> DLADRFAELERRYDARLGVYVPATGTTAAIEYRADERFAFCSTFKAPLVAAVLHQNPLTHLDKLITYTSDDIRGISPVAQQHVQTGMTIGQLCDAAIRYSDGTAANLLLADLGGPGGGTAAFTGYLRSLGDTVSRLDAEESELNRAPPGDERDTTTPHAIALVLQQLVLGNALPPDKRALLTDWMARNTTGAKRIRAGFPADWKVIDKTGTGGYGRANDIAVVWSPTGVPYVVAVMSDRAGGGYDAEPREALLAEAATCVAGVLA

BlaC is a class A serine β‐lactamase found in Mycobacterium tuberculosis (Wang et al., 2006). The enzymes in this class utilize an active site serine (Ser70) to perform a nucleophilic attack on β‐lactam rings, forming a covalent acyl‐enzyme intermediate that is subsequently hydrolyzed (Fisher & Mobashery, 2009; Strynadka et al., 1992). BlaC can efficiently hydrolyze penicillin antibiotics but has low activity against later‐generation oxyimino‐cephalosporins, such as ceftazidime, due to their bulky C7β aminothiazole‐oxyimino side chain (Sun et al., 2023; Wang et al., 2006). We analyzed the structural changes in mutants of the β‐lactamase BlaC from Mycobacterium tuberculosis obtained via directed evolution for increased ceftazidime hydrolysis activity.

The crystal structures of BlaC variants PD, PDDS, and PDDSH were solved at 1.3, 1.6, and 1.4 Å resolution, respectively. Between these mutants, significant differences are observed in the Ω‐loop. In PDDS (blue), the loss of the negatively charged carboxyl group of Asp172 (to Ala) causes disruption of the low‐barrier H‐bond of D179‐D172, which was shown before to stabilize the Ω‐loop in WT BlaC (Sun et al., 2024). As a consequence, the chain between residues 167 and 172 is only partially ordered, indicating mobility in this region of the Ω‐loop. The initial mutations found in the selection screens are located in or close to the Ω‐loop (P167S, D240G), and also in later rounds such mutations were found (D172A, D176G). Also, two mutations in the gatekeeper loop were found (S104G and I105F). As the name suggests, this loop covers part of the entry to the active site and lies over the Ω‐loop (Feiler et al., 2013), and these mutations further enhance the accessibility of the active site (Poirel et al., 2001; Radojković & Ubbink, 2024; Yi et al., 2012). Some mutations stabilize a single conformation, largely eliminating the peak doubling (D172A), and others stabilize one part of the protein and introduce new peak doubling and, consequently, new conformational states, in other regions (H184R). For one branch of the directed evolution experiment, we managed to obtain crystal structures of the successive mutants, PD, PDDS, and PDDSH, showing the opening and increasing disorder of the Ω‐loop in an otherwise defined protein structure, suggesting minor structural changes.>[2x]MDFKYTEAKETIKFNNFMIHKYTVLYTSNCIMDIYSEEEKITCFSNRLVFLERGVNISVRMQKQILSEKPYVAFRLNGDMLRHLKDALMIIYGMSKIDTNACRSMSRKIMTTEVNKTLLDELKNINSHDNSAFISSLIYLISKLENNEKIIESIYISSVSFFSDKVRNLIEKDLSRKWTLGI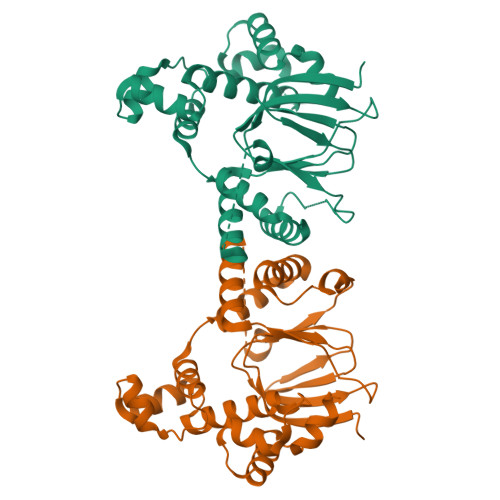IADAFNASEITIRKRLESENTNFNQILMQLRMSKAALLLLENSYQISQISNMIGISSASYFIRIFNKHYGVTPKQFFTYFKGG> NPVENYIDSVL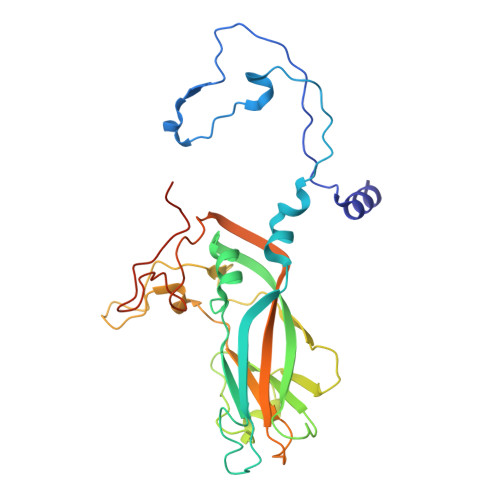NEVLVVPNIQPSTSVSSHAAPALDAAETGHTSSVQPEDMIETRYVITDQTRDETSIESFLGRSGCIAMIEFNTSSDKTEHDKIGKGFKTWKVSLQEMAQIRRKYELFTYTRFDSEITIVTAAAAQGNDSGHIVLQFMYVPPGAPVPEKRDDYTWQSGTNASVFWQEGQPYPRFTIPFMSIASAYYMFYDGYDGDSAASKYGSVVTNDMGTICVRIVTSNQKHDSNIVCRIYHKAKHIKAWCPRPPRAVAYQHTHSTNYIPSNGEATTQIKTRPDVFTVTNVGPSSMF> MPRVVPDQRSKFENEEFFRKLSRECEIKYTGFRDRPHEERQTRFQNACRDGRSEIAFVATGTNLSLQFFPASWQGEQRQTPSREYVDLEREAGKVYLKAPMILNGVCVIWKGWID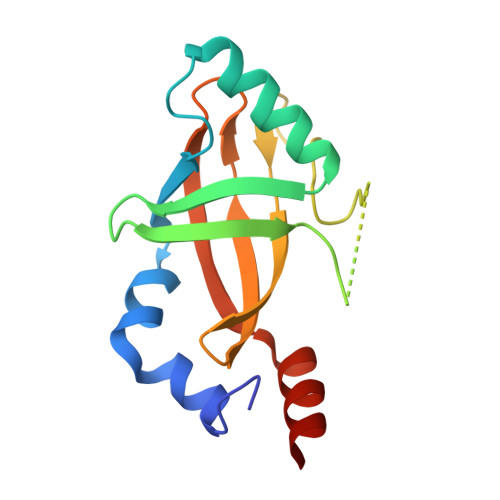LHRLDGMGCLEFDEERAQQEDALAQQA> MGSDKIHHHHHHMKVTVTTLELKDKITIASKALAKKSVKPILAGFLFEVKDGNFYICATDLETGVKATVNAAEISGEARFVVPGDVIQKMVKVLPDEITELSLEGDALVISSGSTVFRITTMPADEFPEITPAESGITFEVDTSLLEEMVEKVIFAAAKDEFMRNLNGVFWELHKNLLRLVASDGFRLALAEEQIENEEEASFLLSLKSMKEVQNVLDNTTEPTITVRYDGRRVSLSTNDVETVMRVVDAEFPDYKRVIPETFKTKVVVSRK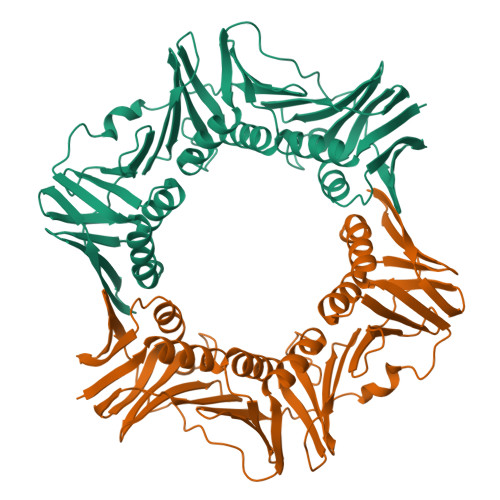ELRESLKRVMVIASKGSESVKFEIEENVMRLVSKSPDYGEVVDEVEVQKEGEDLVIAFNPKFIEDVLKHIETEEIEMNFVDSTSPCQINPLDISGYLYIVMPIRLA P1-P2-METHYLENE-P3-THIO-DIADENOSINE TRIPHOSPHATE | C21 H29 N10 O14 P3 S | 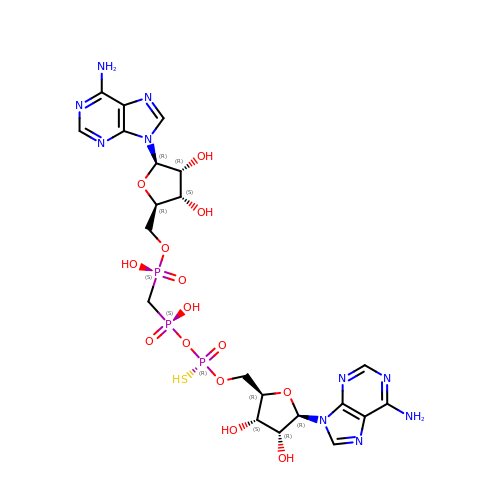UJCWOSLCGXVJOD-LCHUORCTSA-N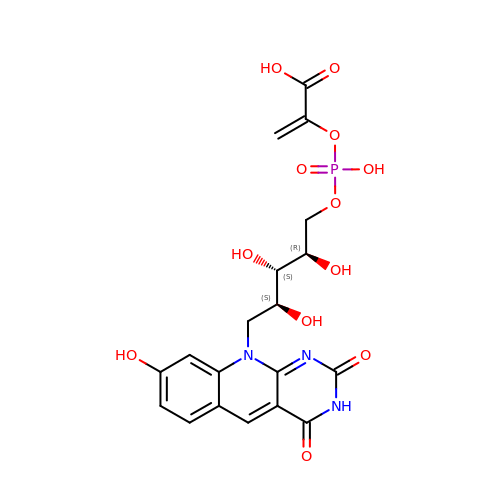2-[oxidanyl-[(2~{R},3~{S},4~{S})-2,3,4-tris(oxidanyl)-5-[2,4,8-tris(oxidanylidene)-1,9-dihydropyrimido[4,5-b]quinolin-10-yl]pentoxy]phosphoryl]oxyprop-2-enoic acid | C19 H20 N3 O12 P | QMXZMTIOXGWNQW-ZNMIVQPWSA-N>[2x]MHRSPLAWLRLLLAAVLGAFLLGGPLHAAETAATRSPAWAQAVDPSINLYRMSPTLYRSALPNAQSVALLQRLQVKTVVSFIKDDDRAWLGQAPVRVLSLPTHADRVDDAEVLSVLRQLQAAEREGPVLMHSKHGNNRTGLFAAMYRIVVQGWDKQAALEEMQHGGFGDEDDMRDASAYVRGADVDGLRLAMANGECSPSRFAVCHVREWMAQALDRP

TpbA is a dual specific tyrosine phosphatase (DUSP) that has a conserved tyrosine phosphatase domain, and relevant phosphatase activities with p-nitrophenyl phosphate (pNPP) and phosphotyrosine peptides have been reported. TpbA (PA3885) from P. aeruginosa PA14 has been reported to be secreted to the periplasm and to link the extracellular quorum-sensing signals to EPS (extracellular polysaccharide) production and biofilm formation via negative regulation of c-di-GMP (3',5'-cyclic diguanylic acid), which regulates biological processes including motility and biofilm formation in bacteria. TpbA adopts a canonical eukaryotic-like DUSP fold with additional secondary structure elements that distinguish it from other DUSPs, including an N-terminal β-strand β0 that caps and extends the β-sheet, and a C-terminal helix α6 that packs on the outside of the protein. The active site architecture of the DUSP catalytic domain is defined by four loops: the protein tyrosine phosphatase (PTP) loop containing the conserved catalytic cysteine Cys132; the general acid loop containing a conserved aspartic acid that functions as a catalytic acid/base; a variable insert that varies among DUSPs and is predicted to involve in substrate recognition; and the α4-α5 loop that is equivalent to the Q-loop in protein tyrosine phosphatases (PTPs).

In an attempt to provide a structural basis for the phosphatase mechanism, we co-crystallised a C132S mutant of TpbA with pTyr on the basis that a C132S mutant of TpbA was previously reported to be inactive by Koveal and colleagues. The TpbA C132S mutant co-crystallized with pTyr shares the same crystal form as native TpbA with two molecules in the a.s.u. Comparison between the wild-type and C132S-pTyr structures reveal an r.m.s.d. of 0.35 Å for 162 aligned Cα atoms, indicating no major differences between the two structures. Close inspection of the electron density maps for the C132S-pTyr structure revealed phosphate alone was present in the active site. In one of the two monomers, however, clear electron density was visible for tyrosine in the shallow binding pocket approximately 5 Å from the bound phosphate, indicating that pTyr had been dephosphorylated. The tyrosine is trapped close to the active site, and its position overlaps with that of a glycerol molecule in the wild-type structure. The trapped tyrosine stacks adjacent to His76 and is coordinated by a 3.1 Å hydrogen bond between the carbonyl oxygen and the amide group of Ala104, and a 2.5 Å hydrogen bond between the amide group and the side chain of Asp175. The side chain of Asp105, the proposed general acid/base, is approximately 3.8 Å from the amide group of the trapped tyrosine, and a weak electrostatic interaction (3.6 Å) is provided between the carbonyl oxygen and the Nε atom of Arg138.> SNAMTNMKLKFDLLLKSYHLSHRFVYKANPGNAGDGVIASATYDFFERNALTYIPYRDGERYSSETDILIFGGGGNLIEGLYSEGHDFIQNNIGKFHKVIIMPSTIRGYSDLFINNIDKFVVFCRENITFDYIKSLNYEPNKNVFITDDMAFYLDLNKYLSLKPVYKKQANCFRTDSESLTGDYKENNHDISLTWNGDY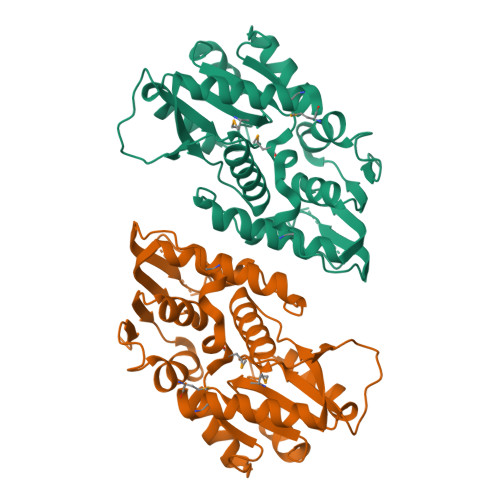WDNEFLARNSTRCMINFLEEYKVVNTDRLHVAILASLLGKEVNFYPNSYYKNEAVYNYSLFNRYPKTCFITAS>[2x]KLEGAFAKGTNVLMADGSIECIENIEVGNKVMGKDGRPREVIKLPRGRETMYSVVQKSQHRAHKSDSSREVPELLKFTCNATHELVVRTPRSVRRLSRTIKGVEYFEVITFEMGQKKAPDGRIVELVKEVSKSYPISEGPERANELVESYRKASNKAYFEWTIEA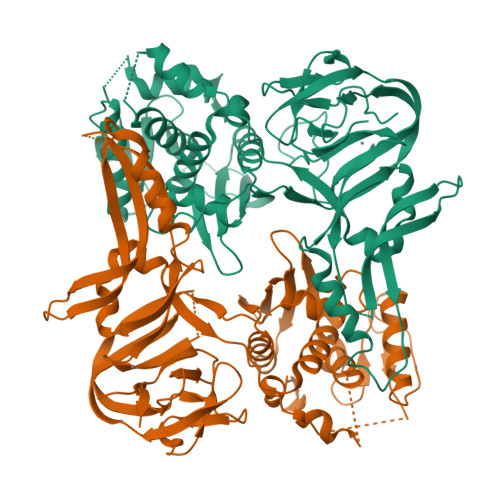RDLSLLGSHVRKATYQTYAPILYENDHFFDYMQKSKFHLTIEGPKVLAYLLGLWIGDGLSDRATFSVDSRDTSLMERVTEYAEKLNLCAEYKDRKEPQVAKTVNLYSKVVRGNGIRNNLNTENPLWDAIVGLGFLKDGVKNIPSFLSTDNIGTRETFLAGLIDSDGYVTDEHGIKATIKTIHTSVRDGLVSLARSLGLVVSVNAEPAKVDMNGTKHKISYAIYMSGGDVLLNVLSKCAGSKKFRPAPAAAFARECRGFYFELQELKEDDYYGITLSDDSDHQFLLANQVVVHACGER> DPLTRVYAKDHFLRLLSYQHQRAFEENTPYTIFFVKTKVSKNEREKALMKIGKILKECVRVPLDSVGRYSDDTFALFVIGVGK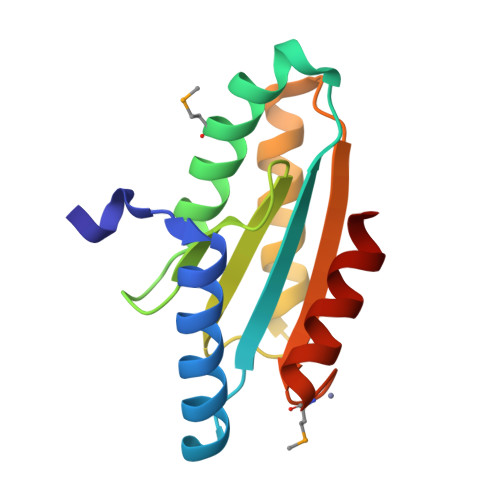ETAPNIEERIKNHIESIGGIEYSIAYKSYPEDFMDLEKAILDLEKAVA>CCAXGCG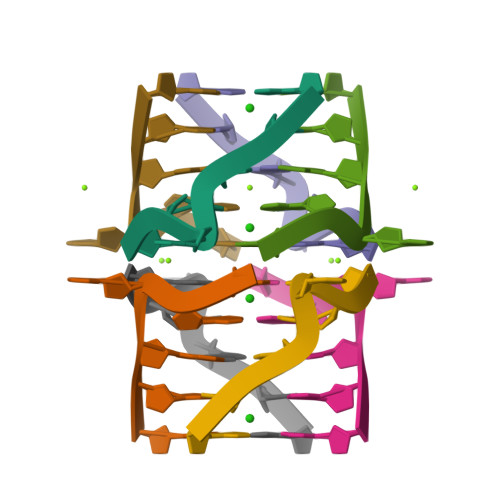TGG[2x]(4S)-6-bromo-3,4-dihydro-2H-thiochromen-4-yl 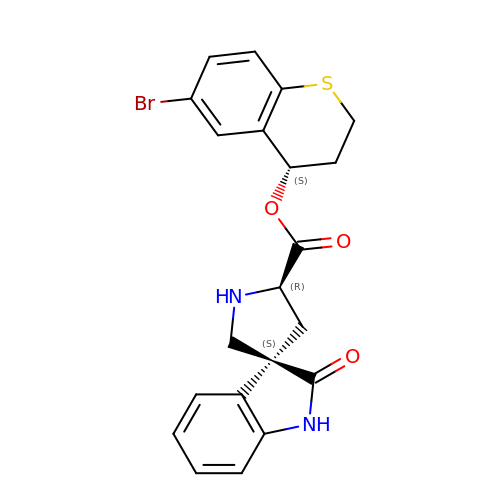(3S,5'R)-2-oxo-1,2-dihydrospiro[indole-3,3'-pyrrolidine]-5'-carboxylate | C21 H19 Br N2 O3 S | OPUJSFZMYKHRTH-LLGFUMIMSA-N>MGSSHHHHHHSSGLEVLFQGPAMATKKVHIISHSHWDREWYMAYEQHHMRLINLIDDLLEVFQTDPDFHSFHLDGQTIILDDYLKVRPEREPEIRQAIASGKLRIGPFYILQDDFLTSSESNVRNMLIGKEDCDRWGASVPLGYFPDTFGNMGQTPQLMLKAGLQAAAFGRGIRPTGFNNQVDTSEKYSSQFSEISWQGPDNSRILGLLFANWYSNGNEIPTTEAEARLFWDKKLADAERFASTKHLLMMNGCDHQPVQLDVTKAIALANQLYPDYEFVHSCFEDYLADLADDLPENLSTVQGEITSQETDGWYTLANTASARIYLKQANTRVSRQLENITEPLAAM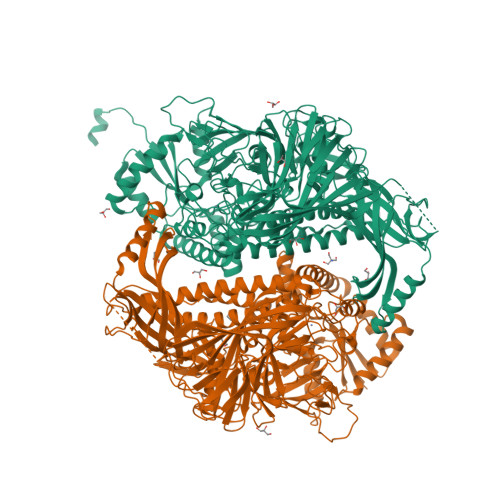AYEVTSTYPHDQLRYAWKTLMQNHPHDSICGCSVDSVHREMMTRFEKAYEVGHYLAKEAAKQIADAIDTRDFPMDSQPFVLFNTSGHSKTSVAELSLTWKKYHFGQRFPKEVYQEAQEYLARLSQSFQIIDTSGQVRPEAEILGTSIAFDYDLPKRSFREPYFAIKVRLRLPITLPAMSWKTLALKLGNETTPSETVSLYDDSNQCLENGFLKVMIQTDGRLTITDKQSGLIYQDLLRFEDCGDIGNEYISRQPNHDQPFYADQGTIKLNIISNTAQVAELEIQQTFAIPISADKLLQAEMEAVIDITERQARRSQEKAELTLTTLIRMEKNNPRLQFTTRFDNQMTNHRLRVLFPTHLKTDHHLADSIFETVKRPNHPDATFWKNPSNPQHQECFVSLFDGENGVTIGNYGLNEYEILPDTNTIAITLLRSVGEMGDWGYFPTPEAQCLGKHSLSYSFESITKQTQFASYWRAQEGQVPVITTQTNQHEGTLAAEYSYLTGTNDQVALTAFKRRLADNALITRSYNLSNDKTCDFSLSLPNYNAKVTNLLEKDSKQSTPSQLGKAEILTLAWKKQ[2x]> MLSYRHSFHAGNHADVLKHTVQSLIIESLKEKDKPFLYLDTHAGAGRYQLGSEHAERTGEYLEGIARIWQQDDLPAELEAYINVVKHFNRSGQLRYYPGSPLIARQLLREQDSLQLTELHPSDYPLLRSEFQKDSRARVEKADGFQQLKAKLPPVSRRGLILIDPPYEMKTDYQAVVSGIAEGYKRFATGTYALWYPVVLRQQIKRMIHDLEATGIRKILQIELAVLPDSDRRGMTASGMIVINPPWKLEQQMNNVLPWLHSKLVPAGTGHATVSWIVPE

We previously designed adenosine-SAM bisubstrate analogues that contain the SAM cofactor with the S-atom replaced by a N-atom directly linked to an adenosine at the point of nucleophilic attack to mimic the substrate/cofactor bound state. These molecules were used to study the substrate recognition of the m6A MTase RlmJ, the Ribosomal RNA large subunit methyltransferase J that N6-methylates the adenine A2030 of the E. coli 23S rRNA. m6A RNA methyltransferases (MTases) catalyze the transfer of the methyl group from the cofactor S-adenosyl-L-methionine (SAM) to the N6-atom of adenines at specific positions in RNA, releasing the cofactor product S-adenosyl-l-homocysteine (SAH). Two crystal structures of RlmJ in complex with RNA–SAM conjugates were solved and revealed the RNA-specific recognition elements used by RlmJ to clamp the RNA substrate in its active site.

The structures of RlmJ bound with GA* or GA*A were refined to 2.3 Å and 1.6 Å, respectively. In the RlmJ/GA* structure, the ASAM moiety is superimposable with the RlmJ-bound conformation of SAH, Asub (corresponding to A2030 in the E. coli 23S rRNA) is bound in the presumed substrate binding site, and the neighbouring guanosine (corresponding to G2029 in the E. coli 23S rRNA) binds in a pocket on the surface of RlmJ next to the catalytic site. The N6-atom of Asub is positioned, through the alkyl chain of the linker, at 3.0 Å away from the carbon corresponding to the Cϵ-atom of the methionine moiety in the SAM cofactor. Such a distance, in two non-linked moieties, would allow for an SN2 methyl transfer to the N6-atom. Asub of GA* is involved in an intricate network of interactions with strictly conserved residues of RlmJ that reveals the RlmJ active site. Asub is indeed π-stacked between the aromatic residues, H9 and W195, and is stabilised by hydrogen bonds from its N1- and N3-atoms to the side chains of the K18 and N12 residues, respectively. D164 forms a hydrogen bond of 2.7 Å to ASAM and we propose that a hydrogen bond between D164 and the N6-atom of A2030 would form in the case of the non-alkylated RNA substrate. This hydrogen bond cannot be formed in this structure due to the N6-alkylation of Asub in GA*. Y167 also—along with residues V199, Y173 and P197—provides a hydrophobic surface near the catalytic pocket where the guanosine is positioned. Interestingly, H9 swaps conformation from solvent exposed in the RlmJ/CA structure, to buried in the RlmJ/GA* structure, from where it can π-stack with Asub.> MLNLENKTYVIMGIANKRSIAFGVAKVLDQLGAKLVFTYRKERSRKELEKLLEQLNQPEAHLYQIDVQSDEEVINGFEQIGKDVGNIDGVYHSIAFANMEDLRGRFSETSREGFLLAQDISSYSLTIVAHEAKKLMPEGGSIVATTYLGGEFAVQNYNVMGVAKASLEANVKYLALDLGPDNIRVNAISAGPIRTLSAKGVGGFNTILKEIKERAPLKRNVDQVEVGKTAAYLLSDLSS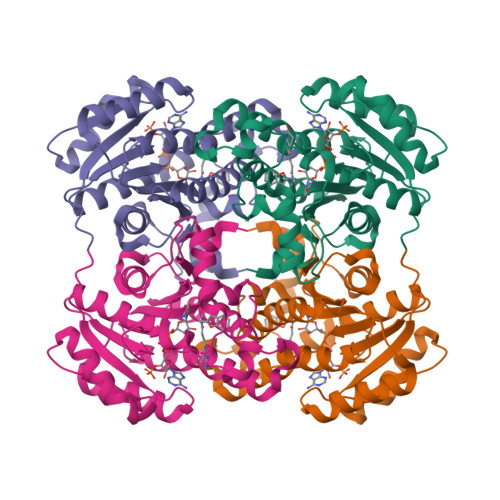GVTGENIHVDSGFHAIK> GSVIDPSELTFVQEIGSGQFGLVHLGYWLNKDKVAIKTIREGAMSEEDFIEEAEVMMKLSHPKLVQLYGVCLEQAPICLVFEFMEHGCLSDYLRTQRGLFAAETLLGMCLDVCEGMAYLEEASVIHRDLAARNCLVGENQVIKVSDFGMTRFVLDDQYTSSTGTKFPVKWASPEVFSFSRYSSKSDVWSFGVLMWEVFSEGKIPYENRSNSEVVEDISTGFRLYKPRLASTHVYQIMNHCWKERPEDRPAFS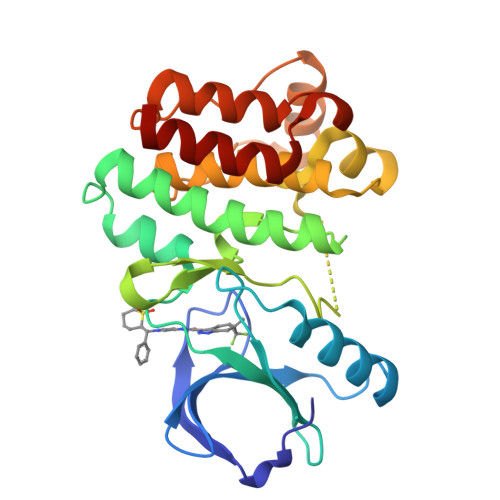RLLRQLAAIAASGL>GSHMASKISDNVRIKLYMEGTVNNHHFMCEAEGEGKPYEGTQMENIKVTKGGPLPFSFDILTPNCQYGSVAITKYTSGIPDYFKQSFPEGFTWERTTIYEDGAYLTTQQETKLDGNCLVYNIKILGCNFPPNG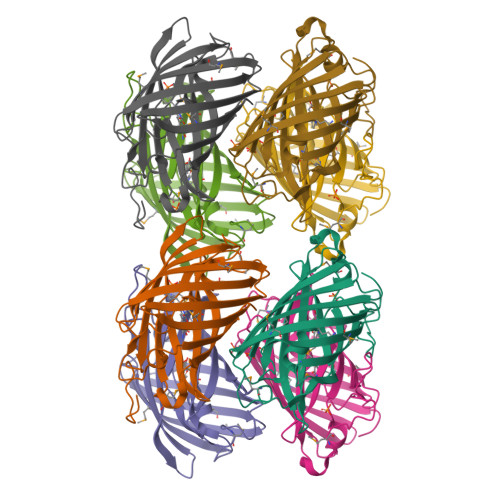PVMQKKTQGWEPCCEMRYTRDGVLCGQTLMALKCADGNHLTCHLRTTYRSKKAAKALQMPPFHFSDHRPEIVKVSENGTLFEQHESSVARYCQTCPSKLGHN[8x]>SNVRATYTVIFKNASGLPNGYDNWGWGCTLSYYGGAMIINPQEGKAGAVSLKRNSGSFRGGSLRFDMKNEGKVKILVENSEADEKFEVETISPSDEYVTYILDVDFDLPFDRIDFQDAPGNGDRI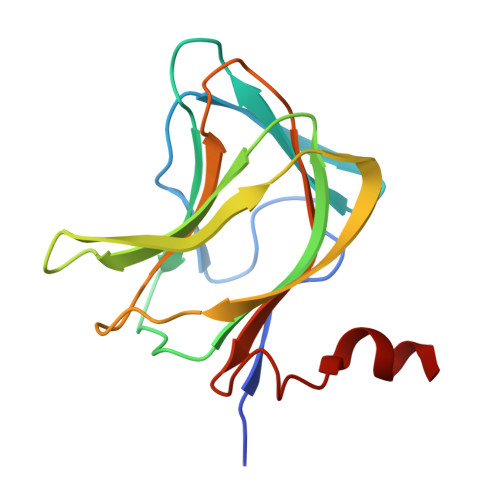WIKNLVHSTGSADDFVDPINLEHH[2x]2-deoxy-2-fluoro-beta-D-glucopyranuronic acid | C6 H9 F O6 | 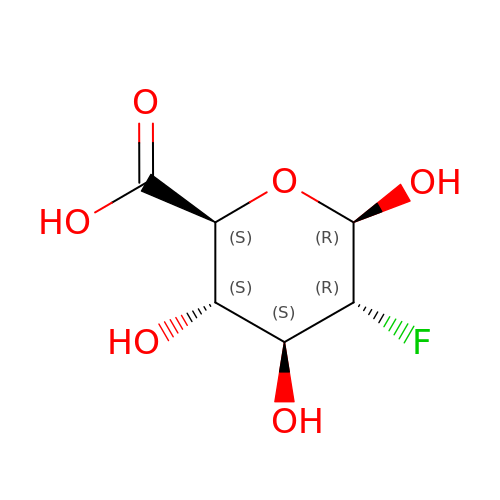LDVYRSUUUDDWHG-LVBGKUAWSA-N> MKKEKIDLFYGALLHNIGKVIQRATGERKKHALVGADWFDEIADNQVISDQIRYHMANYQSDKLGNDHLAYITYIADNIASGVDRRQSNEESDEDTSAKIWDTYTNQADIFNVFGAQTDKRYFKPTVLNLKSKPNFASATYEPFSKGDYAAIATRIKNELAEFEFNQVQIDSLLNLFEATLSFVPSSTNTKEIADISLADHSRLTAAFALAIYDYLEDKGRHNYKEDLFTKVSAFYEEEAFLLASFDLSGIQDFIYNINIATNGAAKQLKARSLYLDFMSEYIADSLLDKLGLNRANMLYVGGGHAYFVLANTEKTVETLVQFEKDFNQFLLANFQTRLYVAFGWGSFAAKDIMSELNSPESYRQVYQKASRMISKKKISRYDYQTLMLLNRGGKSSERECEICHSVENLVSYHDQKVCDICRGLYQFSKEIAHDHFIITENEGLPIGPNACLKGVAFEKLSQEAFSRVYVKNDYKAGTVKATHVFVGDYQCDEIYNYAALSKNENGLGIKRLAVVRLDVDDLGAAFMAGFSQQGNGQYSTLSRSATFSRSMSLFFKVYINQFASDKKLSIIYAGGDDVFAIGSWQDIIAFTVELRENFIKWTNGKLTLSAGIGLFADKTPISLMAHQTGELEEAAKGNEKDSISLFSSDYTFKFDRFITNVYDDKLEQIRYFFNHQDERGKNFIYKLIELLRNHDRMNMARLAYYLTRLEELTRETDRDKFKTFKNLFYSWYTNKNDKDRKEAELALLLYIYEIRKD;>MTILTDENYVDIAEKAILKLERNTRNRKNPDAFFLTTSKLRNLLSLTSTLFDESKVKEYDALLDRIAYLRVQFVYQAGREIAVKDLIEKAQILEALKEIKDRETLQRFCRYMEALVAYFKFYGGKD[2x];>MTFAKIKFSAQIRLETGLHIGGSDAFAAIGAINSPVIKDPITNLPIIPGSSLKGKMRTLLAKVYNEKVAEKPSDDSDILSRLFGNSKDKRFKMGRLIFRDAFLSNADELDSLGVRSYTEVKFENTIDRITAEANPRQIERAIRNSTFDFELIYEITDENENQVEEDFKVIRDGLKLLELDYLGGSGSRGYGKVAFENLKATTVFGNYDVKTLNELLTAEV[3x];> MTYKLYIMTFQNAHFGSGTLDSSKLTFSADRIFSALVLEALKMGKLDAFLAEANQDKFTLTDAFPFQFGPFLPKPIGYPKHDQIDQSVDVKEVRRQAKLSKK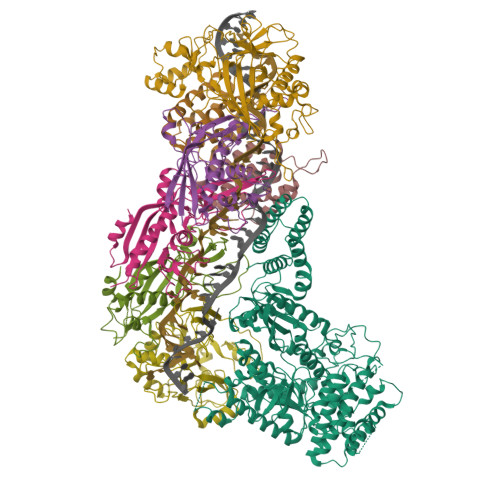LQFLALENVDDYLNGELFENEEHAVIDTVTKNQPHKDDNLYQVATTRFSNDTSLYVIANESDLLNELMSSLQYSGLGGKRSSGFGRFELDIQNIPLELSDRLTKNHSDKVMSLTTALPVDADLEEAMEDGHYLLTKSSGFAFSHATNENYRKQDLYKFASGSTFSKTFEGQIVDVRPLDFPHAVLNYAKPLFFKLEV;> MKNDYRTFKLSLLTLAPIHIGNGEKYTSREFIYENKKFYFPDMGKFYNKMVEKRLAEKFEAFLIQTRPNARNNRLISFLNDNRIAERSFGGYSISETGLESDKNPNSAGAINEVNKFIRDAFGNPYIPGSSLKGAIRTILMNTTPKWNNENAVNDFGRFPKENKNLIPWGPKKGKEYDDLFNAIRVSDSKPFDNKSLILVQKWDYSAKTNKAKPLPLYRESISPLTKIEFEITTTTDEAGRLIEELGKRAQAFYKDYKAFFLSEFPDDKIQANLQYPIYLGAGSGAWTKTLFKQADGILQRRYSRMKTKMVKKGVLKLTKAPLKTVKIPSGNHSLVKNHESFYEMGKANFMIKEIDK> MGSDKIHHHHHHHHHHGVRLGPLWSLPMPGNKGVTGLSESMAPGDIAELGRSAELAFRVRFEGALPPREQLYWRALTMERFDGRRWAQAPQWSGEDALHWQKRGPELRYDVIMQPSSQPWLFALDVAQTDQTDTRLMSDFHLQRRQPVEQRLFYRVSSWPQALRESSIDPRTRWRNLQLPMHGNPRARALADELRQAHAQPQALVAALLQRFNHEPFAYTLKPPATGADGVDDFLFDTRSGFCAHYAGAMAFVLRAAGIPARVVAGYQGGELNPAGNYLLV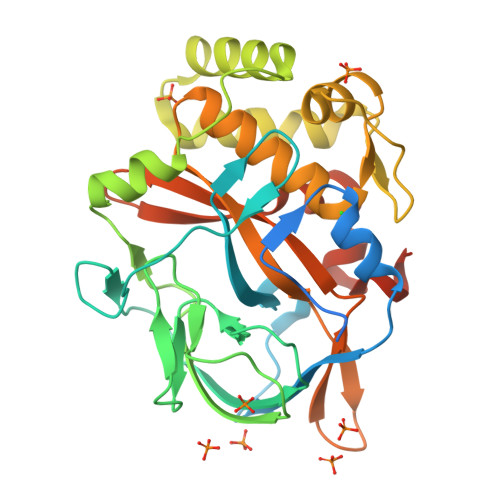HQFDAHAWVEYWQPEQGWLSVDPTYQVAPERIEQGLEQALAGDSEYLADAPLSPLRY>MKKQILFWSMMSWMVSVGLPSFAQTVEDFKPSEVNQPGKLYPQVNSERKVRVQISAPEAKVVQLDLGGVKYDLTKDEKGVWTGESAPQQEGFHYYQLNVDGAAVPDPGTIYFYGAGRWGSGIEVPAHDADFYALKDVPHGLLSEMNYYSNLTKAWRRCFVYTPAGYGDNKDKRYPVLYLQHGSFEDETGWGRQGKTNLILDNLIAAGKAVPMLVVMDNGYATKPGEKSPFAASIFEEVLMNEVIPMIDAKFRTLSGREDRAIAGLSMGANQTMHI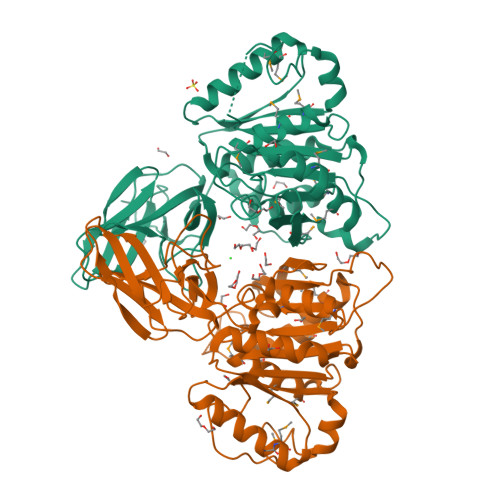AMNNPGHFAYYGGFSGTSNYPSTEPLDATTFLNGKFKDAKAVNVQFKVFFLGLGTAEPHPFPGVVKAFRQMMDKQGIKYVYYESPDTAHEWLTWRRALNEFAPLLFK[2x]3-(4-chlorophenyl)-5-methylsulfanyl-1~{H}-pyrazole-4-carbonitrile 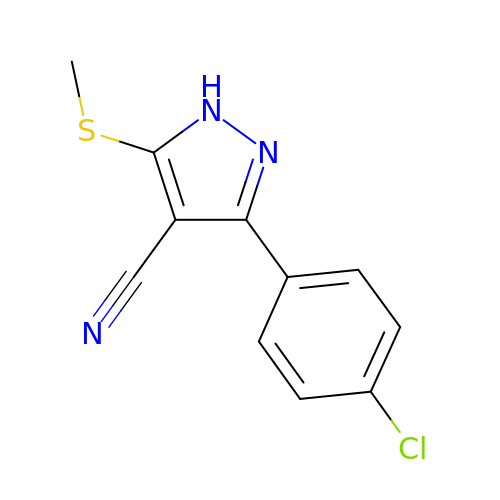| C11 H8 Cl N3 S | KRQSUBRVYHNKPM-UHFFFAOYSA-N> MSELEKAVVALIDVFHQYS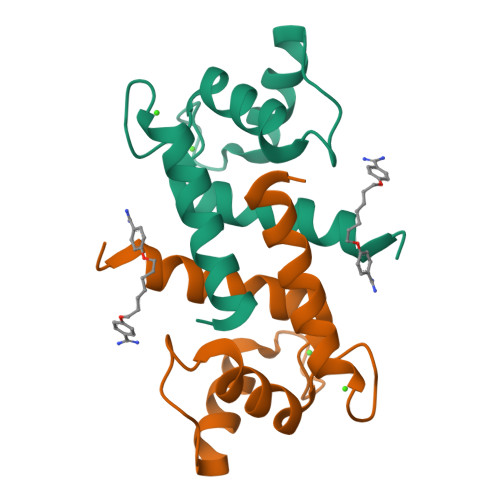GREGDKHKLKKSELKELINNELSHFLEEIKEQEVVDKVMETLDSDGDGECDFQEFMAFVAMITTACHEFF>[2x]MGHHHHHHGSVKIGHYILGDTLGVGTFGKVKVGKHELTGHAVAVKILNRQKIRSLDVVGKIRREIQNLKLFRHPHIIKLYQVISTPSDIFMVMEYVSGGELFDYICKNGRLDEKESRRLFQQILSGVDYCHRHMVVHRDLKP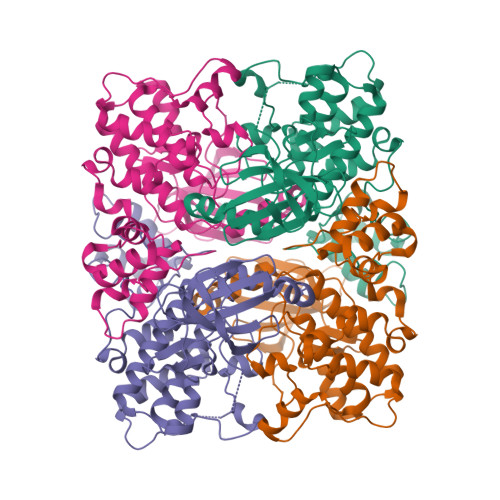ENVLLDAHMNAKIADFGLSNMMSDGEFLRTSCGSPNYAAPEVISGRLYAGPEVDIWSSGVILYALLCGTLPFDDDHVPTLFKKICDGIFYTPQYLNPSVISLLKHMLQVDPMKRASIKDIREHEWFKQDLPKYLFPEDPSYSTTMIDDEALKEVCEKFECSEEEVLSCLYNRNHQDPLAVAYHLIIDNRRIMNEAKDFYLATSPPDSFL The polyamine-binding protein AmvR regulates the multidrug efflux pump AmvA, which is pivotal for transporting polyamines, an abundant and prevalent class of amino acid-derived metabolites. AmvA abundance in vivo is transcriptionally regulated by AmvR, a TetR/AcrR-like regulator that senses cellular polyamine levels and enables the dynamic modulation of amvA expression in response to fluctuating growth conditions. The overall fold change observed in AmvR is characteristic of the TetR/AcrR family of transcription factors and consists of an all-helical regulatory domain (α1–α9). The AmvR protein can be further divided into two subdomains in each protomer: the N-terminal DNA-binding domain (DBD) and the C-terminal ligand-binding domain (LBD).

To understand AmvR’s response mechanism to polyamine, we first determined the crystal structure of an AmvR protein derived from A. baumannii at a resolution of 1.88 Å. A single AmvR polypeptide chain is situated within the asymmetric unit of the crystal and forms a homodimer structure with its corresponding partner in another crystallographic lattice, which is consistent with the results of size-exclusion chromatography. Dimerization occurs primarily through hydrophobic interactions between helices α8 and α9 within the LBD. The second and third helices of the DNA-binding domain exhibit a classical helix-turn-helix (HTH) motif, with the recognition helices (α2) playing a pivotal role in sequence-specific DNA binding and being separated by 55.6 Å in dimeric form (measured as the distance between main-chain carbon atoms of His46). Although the majority of ligand-free and DNA-bound TetR/AcrR-like regulators exhibit distances ranging from 35 to 41 Å, suiting the space between the half-sites in the operator, apo AmvR displays longer distances similar to those usually observed in the ligand-bound state. In its ligand-free state, the DNA-binding domains of the AmvR dimer adopt a dimeric arrangement, maintaining their association, but exhibiting a long distance between the two DNA recognition helices, similar to the arrangement observed in the ligand-bound state. Therefore, we speculated that AmvR may have different states in solution, including apo-state and ligand-bound state, but we only captured one state in the crystal.

> MAYLNRDQRREMILQAAMQIALAEGFTAMTVRRIATEAQTSTGQVHHHFSSASHLKAEAFLKLMEQLDEIEQTLQTTSQFQRLFILLGAENIDRLQPYLRLWNEAELLIEQDIEIQKAYNLAMQSWHQAIVQSIECGQKEGEFKNRSNSTDIAWRLIAFVCGLEGIYKLGLQGLAEEDFKRHTEAIIRLELL> MDIQRVKRLLSITNDKHDEYLTEMVPLLVEFAKDECHNPFIDKDG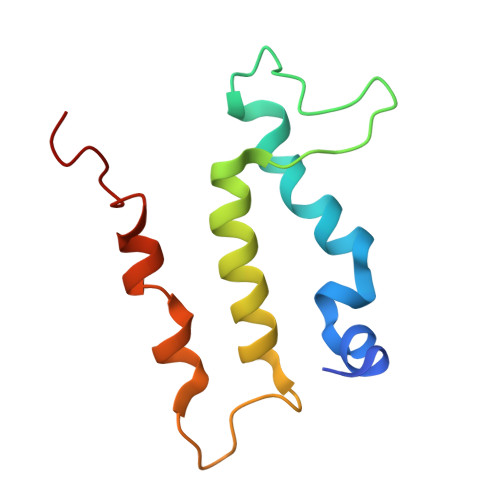NESIPSGVLIFVAKAAQFYMTNAGLTGRSMDTVSYNFATEIPSTILKKLNPYRKMAR>[6x]MAHHHHHHMEFSTKTEILQEQQAGAQLFVCADKAPEHNTAAHALFSALEEGQNFSDTKIPTDNGLQAVAVVRLEKTDRAALNKAAAEAAKWAQNQETVNVDVHAFDEAQAAAVAEAFAIAFGNAAYRFDRYKKEAKPAKFSQAVFHSAHEAAVKEALRVAEAQVYGQS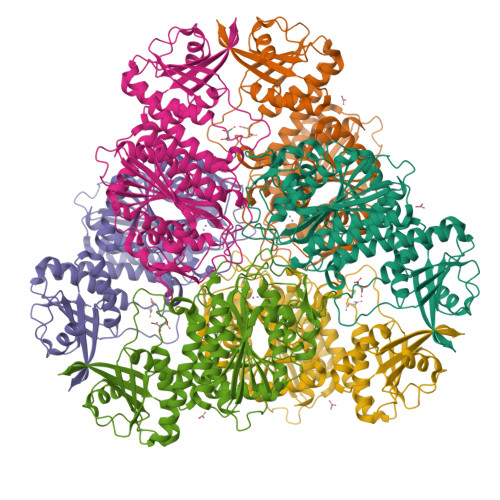LCRDLGNAAPNECTPEFLARTAKAEAEKLGAHAKIIEKDYIKENMGSFWSVAKGSVEDPYLVELSYFGAADKEAAPVVLVGKGITFDTGGISLKPGLNMDEMKFDMCGAATVISTFCAAVKLQLPINLIAIVATCENMPSGAANKPGDVVKSMKGLTIEVLNTDAEGRLILCDALTYAEQFKPKAVIDVATLTGACIVALGHDVSGVMGNNQDLIDSLLAASYNVDDKAWQLPLFETYKDQLKSNFADIPNIGTPGAGTITAATFLSYFTEGYPWAHLDIAGTAWKSGAEKGATGRPVPLLMNYLRNL> SGDYRVQNTSLEAIVQNASSDNQGIQLSAVQAARKLLSSDRNPPIDDLIKSGILPILVHCLERDDNPSLQFEAAWALTNIASGTSEQTQAVVQSNAVPLFLRLLHSPHQNVCEQA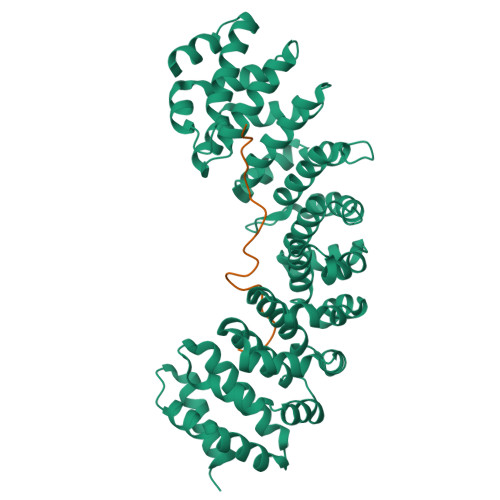VWALGNIIGDGPQCRDYVISLGVVKPLLSFISPSIPITFLRNVTWVMVNLCRHKDPPPPMETIQEILPALCVLIHHTDVNILVDTVWALSYLTDAGNEQIQMVIDSGIVPHLVPLLSHQEVKVQTAALRAVGNIVTGTDEQTQVVLNCDALSHFPALLTHPKEKINKEAVWFLSNITAGNQQQVQAVIDANLVPMIIHLLDKGDFGTQKEAAWAISNLTISGRKDQVAYLIQQNVIPPFCNLLTVKDAQVVQVVLDGLSNILKMAEDEAETIGNLIEECGGLEKIEQLQNHENEDIYKLAYEIIDQFFSSDDIDEDPSLVPEAIQGGTFGFNSSANVPTEGFQF;> SRSLNMLGRKTCLGRRVVQPGMFADYPPTKKARVLLRRMSN>[4x]SHRNEAGHGDLHEILHEAVPLDANEREILELKEDAFAQRRREIETRL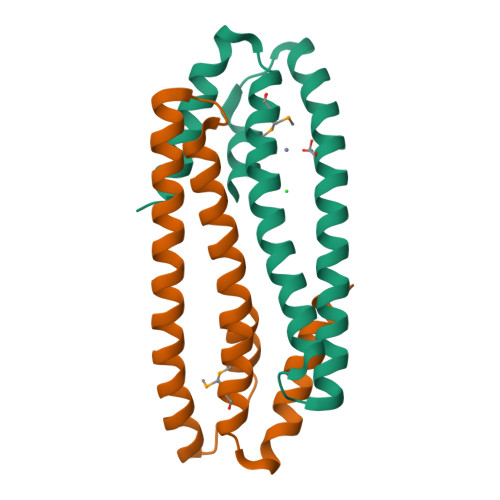RAANGKLADAIAKNPAWSPEVEAATQEVERAAGDLQRATLVHVFEMRAGLKPEHRPAYDRVLIDALRRGSQ>[2x]SHM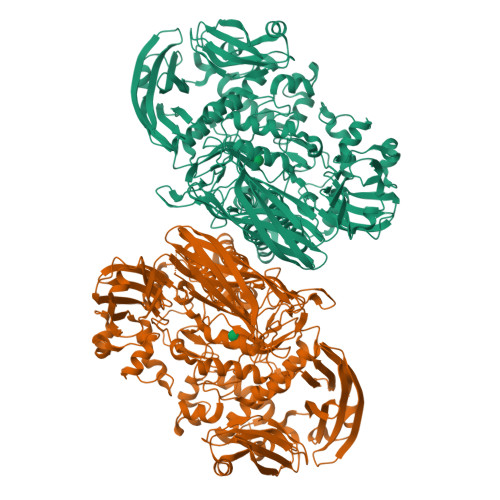TAVTLDGGWRVRLVPGQEQGKTYPKAAAWLPAQVPGAVQTDLIAAKIVPDPFYRDNEGKIQWAGLSDWQYQTRFTVDAATLKREHVELVFDGLDTFAEVTLNGKQLLSADNMFRQWRVDAKSLLKRGDNLLEVKLYSPIKKIQPWLAKQPYALPGAYDSAFGDEPEARHSSTYVRKAPYNFGWDWGPRMVNAGIWKDVRVEAWDAVRVDGLHIAQQRVDAHSAQVQAQLDLQAGRSGPVQVTLDVLGPDGQKVGQFTQDAVVDPGQNRVDLAVRIANPKRWFPAGYGAQDRYTFVASVRDADGDSQQIKRVTGLRSVELRREKDRFGKSMEIVINGIPIFAKGANLIPLDAFPARVTHERMRSTLQDARDANMNMLRMWGGGHYQDDYFYDVADELGIMIWQDFMFGGAVPPYDVEFRENTRQEAIEQVKRLRDHPSLVLWCGNNEVQTGWENWGDRVKFKQSVDPEERTRIERGMTTLFGTVFREVVATYDSDVPYWATSPGTDFDGAADQTNDGDMHYWKVWGGPALPVTEYLNVTPRFMSAYGLQSFPDMRTVRAFAEPGDMDPESPVMRVHQKFDKGNGNKRLMLYIRREFGEPKDFESFVYLSQLMQAEGINIAASHLRASRPQSMGSLYWQLNDVWPGASWSSVDYYGRWKALHYHARRFYAPEMIAALRNDKGQTEVSLVSDRTTPLTARWRMRVMGMDGKVLSKREEKASVNALSSQHVGNFSDKQLLGSADPKRTYAVFELLDGDTLLSREVVFFAPAKQLALPAAKIDSQWRADGDGYALTLTSDTLAREVWLSFGDVDATLSDNAFDLLPGEPLTVRVTSKAALAQLQSALQVRDLAATLAGAPPE>GUCUCCUAG[3x];>CUAGGAGAC[3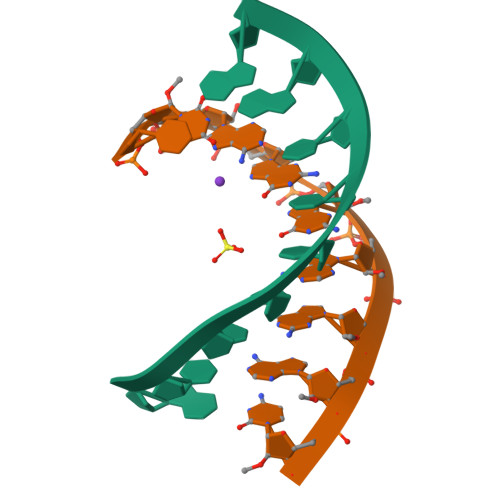x]[(5,7-dimethyl-2-oxo-1,2-dihydroquinolin-4-yl)methyl]phosphonic 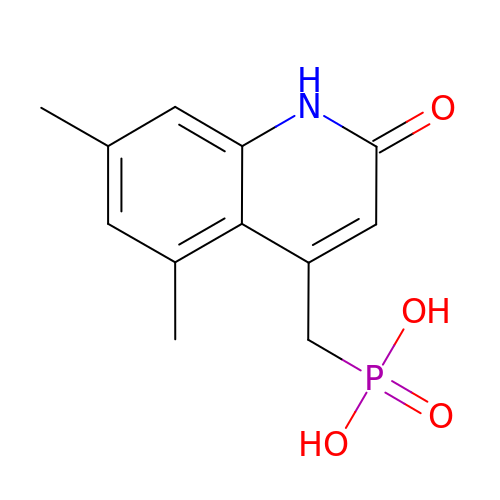acid | C12 H14 N O4 P | HMRCSSLTJXSSFR-UHFFFAOYSA-N(1r,2R,3S,4s,5R,6S)-2,3,4,5,6-pentakis(phosphonooxy)cyclohexyl trihydrogen diphosphate | C6 H19 O27 P7 | 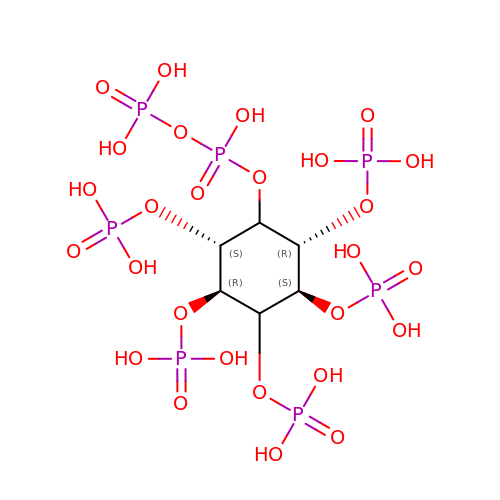UPHPWXPNZIOZJL-KXXVROSKSA-N> MTYNVWNFGESNGRYSALTARGISKETCQKAGYWIAKVDGVMYQVADYRDQNGNIVSQKVRD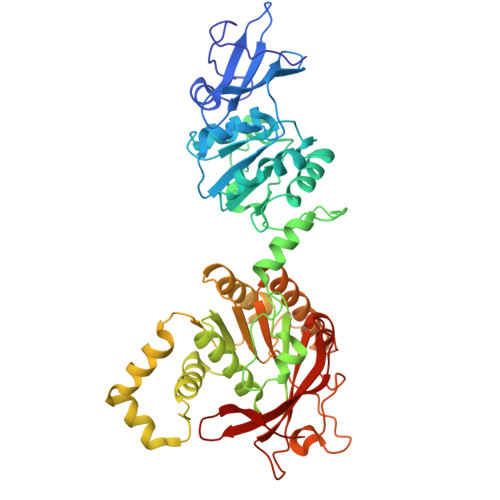KDKNFKTTGSHKSDALFGKHLWNGGKKIVVTEGEIDMLTVMELQDCKYPVVSLGHGASAAKKTCAANYEYFDQFEQIILMFDMDEAGRKAVEEAAQVLPAGKVRVAVLPCKDANECHLNGHDREIMEQVWNAGPWIPDGVVSALSLRERIREHLSSEESVGLLFSGCTGINDKTLGARGGEVIMVTSGSGMGKSTFVRQQALQWGTAMGKKVGLAMLEESVEETAEDLIGLHNRVRLRQSDSLKREIIENGKFDQWFDELFGNDTFHLYDSFAEAETDRLLAKLAYMRSGLGCDVIILDHISIVVSASGESDERKMIDNLMTKLKGFAKSTGVVLVVICHLKNPDKGKAHEEGRPVSITDLRGSGALRQLSDTIIALERNQQGDMPNLVLVRILKCRFTGDTGIAGYMEYNKETGWLEPSSYSG>MPNFSGNWKIIRSENFEELLKVLGVN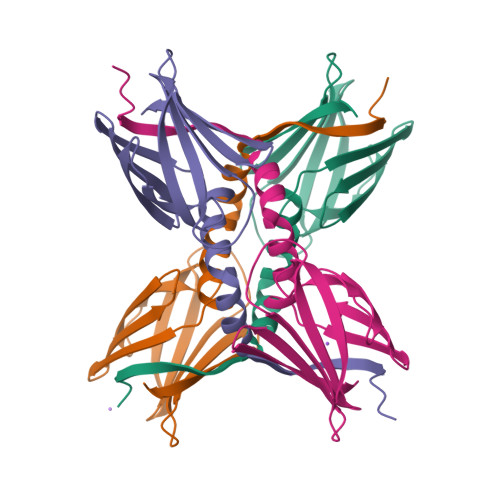VMLAAIAVAAASKPAVEIKQEGDTFYIKTSTTVRTTEINFKVGEEFEEQTVDGRPCKSLVKWESENKMVCEQKLLKGEGPKTSWTRELTNDGELILTMTADDVVCTRVYVRE[4x]>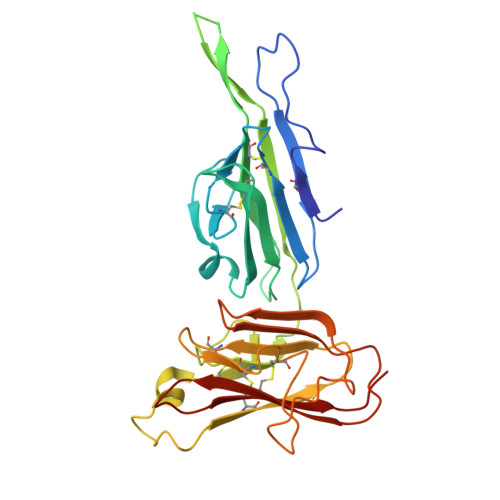 GASNLTCDFNDVYKLEFHPNQQTSVTKLCNLTPNVLEKVTIKCGSDKLNYNLYPPTCFEEVYASRNMMHLKKIKEFVIGSSMFMRRSLTPNKINEVSFRIPPNMMPEKPIYCFCENKKTITINGSNGNPSSKKDIINRGIVEIIIPSLNEKVKGCDFTTSESTIFSKGYSINEISNKSSNNQQDIVCTVKAHANDLIGFKCPSNYSVEPHDCFVSAFNLSGKNENLENKLKLTNIIMDHYNNTFYSRLPSLISDNWKFFCVCSKDNEKKLVFTVEASISS Nucleocytoplasmic protein O-GlcNAcylation is a dynamic modification catalysed by O-GlcNAc transferase (OGT) and reversed by O-GlcNAc hydrolase (OGA), whose activities are regulated through largely unknown O-GlcNAc-dependent feedback mechanisms. OGA is a homodimeric, multi-domain enzyme containing a catalytic core and a pseudo-histone acetyltransferase (pHAT) domain. Here, we show that the eukaryotic OGA pHAT domain forms catalytically incompetent, symmetric homodimers, projecting a partially conserved putative peptide-binding site. In solution, OGA exist as flexible multi-domain dimers, but catalytic core-pHAT linker interactions restrict pHAT positional range.

To determine the spatial arrangement of the pHAT domains relative to the catalytic core, the full-length TaOGA structure was solved by cryo-EM. Initial 2D classification revealed a well-defined homodimeric catalytic core but lacked clear density for the pHAT domains. Subsequent 3D reconstruction produced a map resolving the TaOGA homodimeric catalytic and stalk domains at 3.0 Å resolution, into which an AlphaFold3 model guided model building. The dimerisation interface of TaOGA buries 2700 Å2 of the total 20,000 Å2 surface area, accounting for 14%, as calculated by the PISA server, which is 20% smaller than the reported value for the hOGA crystal structures. The interface is largely conserved, differing at only a few residues, and forms a broad solvent-exposed hollow channel through the homodimer. The top of the stalk domains of this TaOGA cryo-EM structure are in the same tight arrangement as in the hOGA catalytic core crystal structures, whereas one of the TaOGA catalytic domains rotates away from the neighbouring stalk domain, which is reflected in a pairwise inter-Cα distance of 33 Å in TaOGA (Lys59) and 40 Å in hOGA (Val113). The absence of visible pHAT domains in 2D classifications and 3D reconstruction suggests substantial flexibility between the catalytic core and pHAT domains, despite the presence of a short linker (STDEYEESTLKNS) connecting them. Notably, several negative charges in the linker may contribute to electrostatic repulsion of these regions in the homodimer. Taken together, these data suggest that TaOGA, like hOGA, is a homodimer with dimerisation interfaces for the catalytic cores and pHAT domains, although the latter are averaged out due to the flexible linkers under conditions of the cryo-EM experiment. Notably, the linker connecting the catalytic core and the pHAT domain is smaller in TaOGA and not conserved between the two organisms, likely weakening the interaction between the catalytic core and the pHAT domains, resulting in no observed density for the pHAT domains in the cryo-EM structure of TaOGA.

>MTSDKFLSGVVEGFYGKPWSFEQRKTLFSNMAKWGLNTYMYGPKDDEKHRAAWKQAYSKREGDSLRALIRAAEESGILFIYAISPGVDITYSSNRDMKFLKDKLDQIRNFGCNSFAIFFDDIDTVMCLQDQEEFESFAAAQVEVTNEIYKYLGMPANFLFCPTEYCAARADPNVKESKYLVTVGTGLHSDIHIMWTGPKVVSNKISVESILELQTVLRRKPVIWDNIHANDYEQGRLNLGPYDCRPAELMESLNGIFTNPNCEFELNYVPIRTFSLWCQSKRTRFNYDVEKALEQSIREWTEEFCIPRLPDGYLLEADTSDTNVNEYMDDEMQSDSRPISPANSMETDKDELTVKDIRLLVELFYLPQKHGKTANDLLAQAKWLKSNFRIAALSRKPNDTSEGSNLDEHNTDYIAAKEWDKRFSKFRSICQIIHQFGDRLMTCRNRVLLYEVYNYVADLCGILYHLISRIHSLANPEKLEKRSDSEQSSFRYGGFVGDIHRLIVSTDEYEESTLKNSDAYVIRPFMPSDEETLYDLCLKSCIENSNGDEIYKREPRIIGDRDLGAYIYLHPEYIYVLEDDRDKICGYLCGALDSKQFYERYESEWLTQIRDRHPQPENDIASWTPEEIVANSFYNFTPPTDVSVLYLSHLEARFDSSVPEKVIKRIIRFILEQLKAKGSYGASMLIDSWRTNLRRIFTSMGFVDLQEYSWMSEQKCMIAIKLM[2x]> MYGKLLICATASI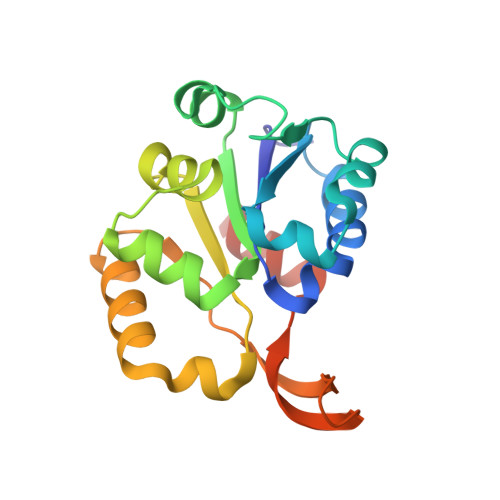NVININHYIVELKQHFDEVNILFSPSSKNFINTDVLKLFCDNLYDEIKDPLLNNINIVENHEYILVLPASANTINKIANGICDNLLTTVCLTGYQKLFIFPNMNIRMWGNPFLQKNIDLLKNNDVKVYSPDMNKSFEISSGRYKNNITMPNIENVLNFVLNNEKRPLD4-{4-[(3R)-3-methylmorpholin-4-yl]-6-[1-(S-methylsulfonimidoyl)cyclopropyl]pyrimidin-2-yl}-1H-indazole | C20 H24 N6 O2 S | 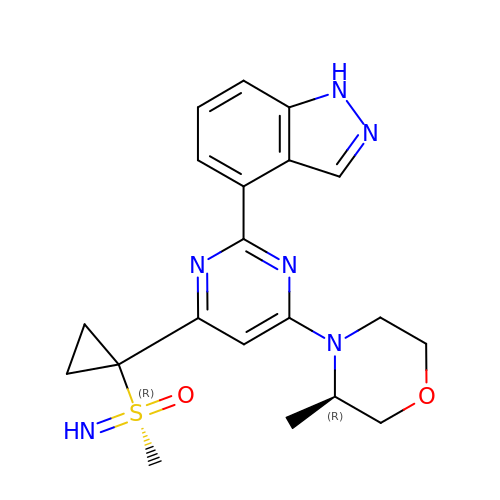RGWFSUWYUBMWFI-JYCIKRDWSA-N>GSEFELACSQGNRTIDLNSLQSTLEKAGPGDTIYIKSGTYTNIQLQLEGYGKVEEPIVVMAQQPGSVFIEGVSNLRLCGEYVEINGLHFRNGYTPKGAVIEFRNGEKVANNCRITDCVIDYFNPIDRGVSGSWILLYGRNNRLDHNSILGKLYAGVTLAVILNGEGDRNNNHRIDHNYFGERPILGSNGGETIRVGTSHHAFFSSNTVIEDNMFHHCNGEVEVVSIKSSDNIIRNNVFLECRGILALRHGNRNLVEGNAFIGNGLPCTGGVRIVNEGHTIKGNLFYGLKGDRFFAALGLMNAVPNSLPNRYHHVKDVTLEDNRFINCDNILFCVGKDNERTLPPSNISFIRNQFISKSDKALYQSFDDISGFTFIDNVVNYPYTVTQRGFQNNTTLSDSIDLKPYMEKKNGASWYTLSENHELVLTGNEISVKAGQNTLLEALNQAQSGDILNLSEEGVYWLDNTLLIDKYIRIQADSHLSKRPVLCFNGMSGKAFVTIVNGGNLEIQGLAFNGEGEAGKALSEGGITVKSGTITPYLLTVDNCEFYNFNESGLAAIRGEKSTFSPMVIIRNSFFHDMSGEAINFAGEKDDKGKYNVEELHVDN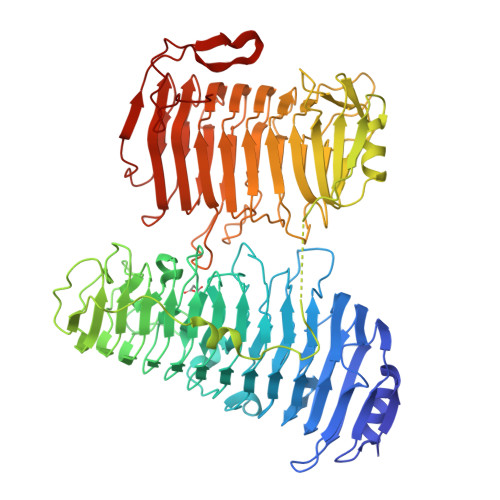CIFYRLLGSALNIYRGGNDESTSGPLLTVDHCTIENVDNKEQGSAMRLIGVQSATVTNCSFANSGKGGASIRFNEMSWDKLSVSYINLYNSGRIASFWGKLGSKNITNYRPEYVDANTGNFYQISTSPLSNKASDKKDLGITQ[4x]>SNAMKYIDCAVIGAGPAGLNASLVLGRARKQIALFDNNTNRNRVTQNSHGFITRDGIKPEEFKEIGLNEVMKYPSVHYYEKTVVMITKQSTGLFEIVTKDHTKYLAE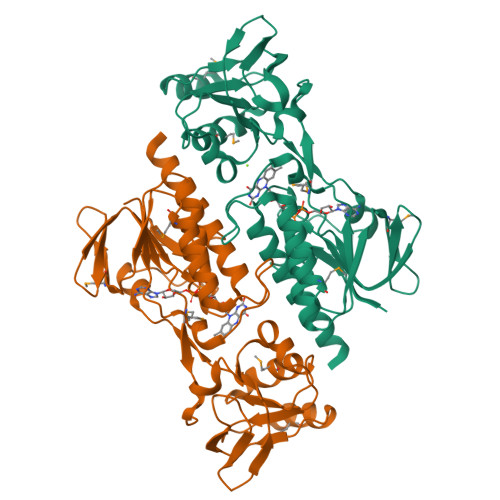RVLLATGMQEEFPSIPNVREYYGKSLFSCPYCDGWELKDQPLIIISENEDHTLHMTKLVYNWSTDLVIATNGNELSQTIMDELSNKNIPVITESIRTLQGEGGYLKKVEFHSGLRIERAGGFIVPTFFRPNQFIEQLGCELQSNGTFVIDDFGRTSEKNIYLAGETTTQGPSSLIIAASQGNKAAIAINSDITDERF[4x]> MAVNDYEPGSMVITHVQGGGRDIIQYIPARSSYGTPPFVPPGPSPYVGTGMQEYRKLRSTLDKSHSELKK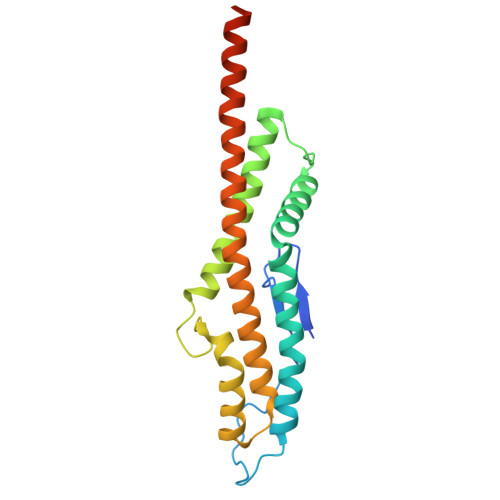NLKNETLKEVDELKSEAGLPGKAVSANDIRDEKSIVDALMDAKAKSLKAIEDRPANLYTASDFPQKSESMYQSQLLASRKFYGEFLDRHMSELAKAYSADIYKAQIAILKQTSQELENKARSLEAEAQRAAAEVEADYKLEHHHHHH> SNATFLELVEVPCNSVHVQGVMTPNQMVKVTGAGWDNGVLEFYVTRPTKTGGDTSRSHLASIMCYSKDIDGVPSDKAGKCFLKRFSGEDSSEID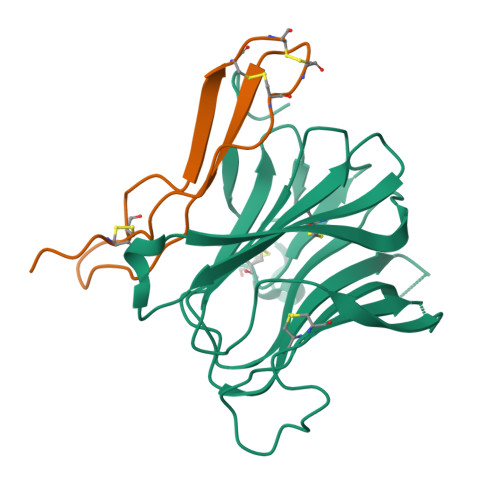EKEVSLPIKSHNDAFMFVCSSNDGSALQCDVFALDNTNSNDGWKVNTVDLGVSVSPDLAFGLTADGVKVKKLYASSGLTAINDDPSLGCKA;> SNAGASCTYVWSDWNKCVCPMGYQARHAAVKFDYRNKPCDLPTFETKACSCGETNPVP> TVGAVALDLDGNLAAATST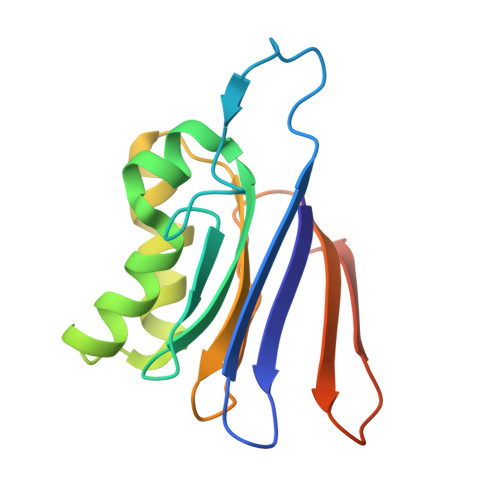GGMTNKLPCTVGAAPLVGAGCYANNASVAVSCTGTGEVFIRALAAYDIAALMDYGGLSLAEACERVVMEKLPALGGSGGLIAIDHEGNVALPFNTEGMYRAWGYAGDTPTTGIYREKGDTVATQ> MAHHHHHHMENLYFQGMSSFLPEGGCYELLTVIGKGFEDLMTVNLARYKPTGEYVTVRRINLEACSNEMVT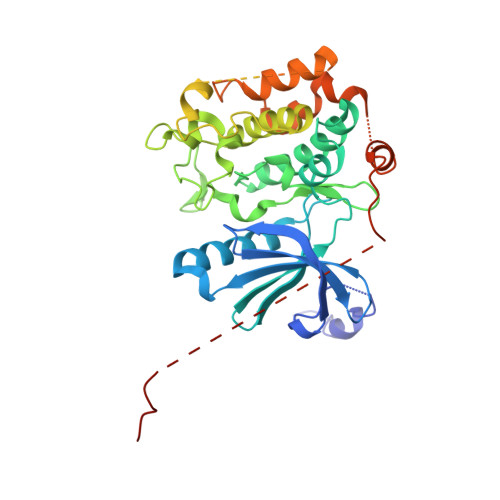FLQGELHVSKLFNHPNIVPYRATFIADNELWVVTSFMAYGSAKDLICTHFMDGMNELAIAYILQGVLKALDYIHHMGYVHRSVKASHILISVDGKVYLSGLRSNLSMISHGQRQRVVHDFPKYSVKVLPWLSPEVLQQNLQGYDAKSDIYSVGITACELANGHVPFKDMPATQMLLEKLNGTVPCLLDTSTIPAEELTMSPSRSVANSGLSDSLTTSTPRPSNGDSPSHPYHRTFSPHFHHFVEQCLQRNPDARPSASTLLNHSFFKQIKRRASEALPELLRPVTPITNFEGSQSQDHSGIFGLVTNLEELEVDDWEF4-(4-CHLOROPHENYL)IMIDAZOLE | C9 H7 Cl N2 | 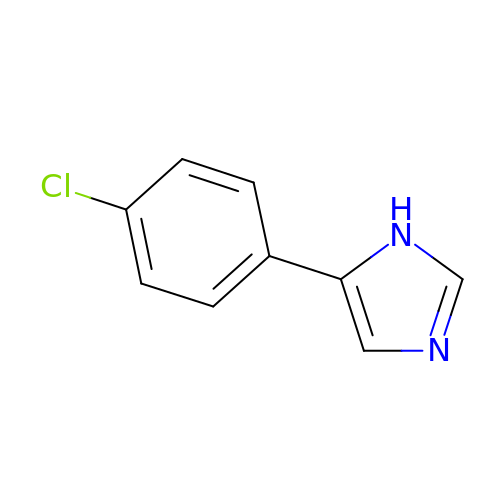DVKIFCXVRCGAEE-UHFFFAOYSA-N>MGHHHHHHGNITLTKRQQEFLLLNGWLQLQCGHAERACILLDALLTLNPEHLAGRRCRLVALLNNNQGERAEKEAQWLISHDPLQAGNWLCLSRAQQLNGDLDKARHAYQHYLELKDHNESP[2x];>GAMALLPDGQSIEPHISRLYPERLADRALLDFATPHRGFHDLLRPVDFHQAMQGLRSVLAEGQSPELRAAAILLEQMHADEQLMQMTLHLLHKV[2x]

SctX proteins are secreted substrates and are essential components of type III secretion systems. The dedicated chaperone SctY escorts SctX proteins to the secretion machinery, where the hydrophobic helix at the C-terminus of SctX mediates recognition by the export apparatus. The type III secretion substrate SctX binds its chaperone at two distinct sites: (i) its α1 helix interacts with the concave groove of SctY and (ii) the two C-terminal helices α2 and α3 cover the large hydrophobic surface formed by the N-terminal TPR of the chaperone.

We co-purified and crystallized two different complexes of AscX and YscY, with the substrate truncated N-terminally to residue 30 (AscX31) or residue 48 (AscX49). The AscX31–YscY complex crystallized with two almost identical complexes in the asymmetric unit. Despite AscX containing all amino acids after residue 30, the electron density only supported model building from Arg45, indicating that the N-terminus is disordered. Superimposing the YscY monomers using LSQKAB revealed a purely rotational relation between the two chains, with an angle of 90.1° between the twofold axis and the centroid vector and a rotation of χ = 179.0°. Furthermore, AscX31–YscY did not show oligomerization when subjected to gel filtration, where it eluted as a single peak at the retention volume expected for a 1:1 heterodimer. Interestingly, both AscX monomers showed a bend in the α3 helix at Ala106 despite the high propensity of alanine for the formation of helices. The α3 kink observed in the two AscX structures allows approximately the last 15 residues of the substrate to fold back onto a hydrophobic patch on helix α1 of SctY. Consequently, the hydrophobic SctV-binding C-terminus of SctX is shielded by a hydrophobic patch on SctY instead of protruding from the chaperone. An extended C-terminus of AscX would not fit into this configuration of the proteins, hence the α3 kink facilitates the assembly of the disulfide-bridged heterotetramer in the asymmetric unit of the AscX31–YscY crystals. In AscX31–YscY, the distance between the phenylalanine side chain and the terminal methyl group of Met79 amounts to 3.9 Å.> SENSVETQEITTFHDVETPNRIDTPMAQDTSSARNMDDTHSIIQFLQRPVLIDNIEIIAGTTADANKPLSRYVLDQQNSQKYVRSWTLPSTVLRAGGKAQKLANFKYLRCDVQVKLVLNANPFVAGRMYLAYSPYDDKVDTARSVLQTSRAGVTGYPGVELDFQLDNSVEMTIPYASFQEAYDLVTGTEDFVQL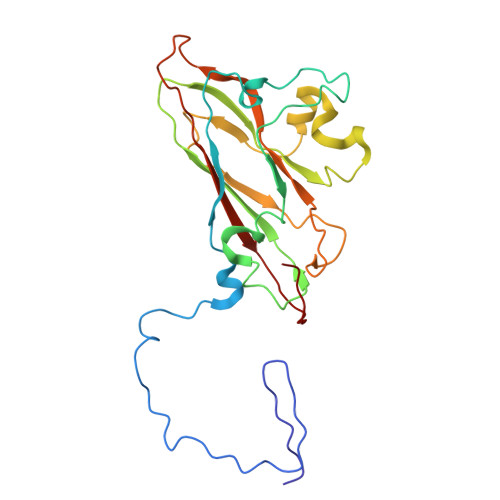YLFPITPVLGPKSESESSKVDISVYMWLSNISLVIPTYRINP> RTIRYVRYESELQMPDIMRLITKDLSEPYSIYTYRYFIHNWPQLCFLAMVGEECVGAIVCKLDMHKKMFRRGYIAMLAVDSKYRRNGIGTNLVKKAIYAMVEGDCDEVVLETEITNKSALKLYENLGFVRDKRLFRYYLNGVDALRLKLWLR;> NWVDITQDFEEACRELKLGELLHDKLFG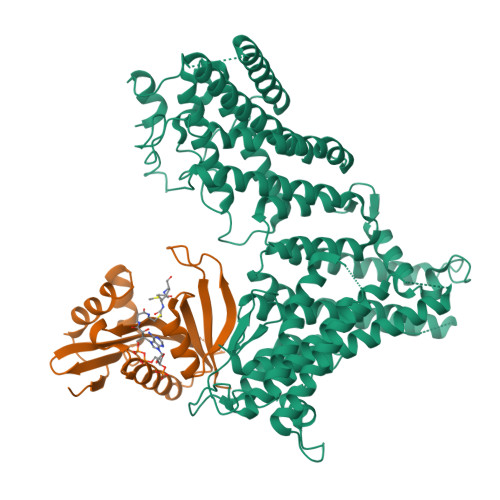LFEAMSAIEMMDPKMDAGMIGNQVNRKVLNFEQAIKDGTIKIKDLTLPELIGIMDTCFCCLITWLEGHSLAQTVFTCLYIHNPDFIEDPAMKAFALGILKICDIAREKVNKAAVFEEEDFQSMTYGFKMANSVTDLRVTGMLKDVEDDMQRRVKSTRSRQGEERDPEVELEHQQCLAVFSRVKFTRVLLTVLIAFTKKETSAVAEAQKLMVQAADLLSAIHNSLHHGIQAQNDTTKGDHPIMMGFEPLVNQRLLPPTFPRYAKIIKREEMVNYFARLIDRIKTVCEVVNLTNLHCILDFFCEFSEQSPCVLSRSLLQTTFLVDNKKVFGTHLMQDMVKDALRSFVSPPVLSPKCYLYNNHQAKDCIDSFVTHCVRPFCSLIQIHGHNRARQRDKLGHILEEFATLQDEAEKVDAALHTMLLKQEPQRQHLACLGTWVLYHNLRIMIQYLLSGFELELYSMHEYYYIYWYLSEFLYAWLMSTLSRADGSQMAEERIMEEQQKGRSSKKTKKKKKVRPLSREITMSQAYQNMCAGMFKTMVAFDMDGKVRKPKFELDSEQVRYEHRFAPFNSVMTPPPVHYLQFKEMSDLNKYSPPPQSPELYVAASKHFQQAKMILENIPNPDHEVNRILKVAKPNFVVMKLLAGGHKKESKVPPEFDFSAHKYFPVVKLV> GSQVQTNVRCQGGSCASVCRRE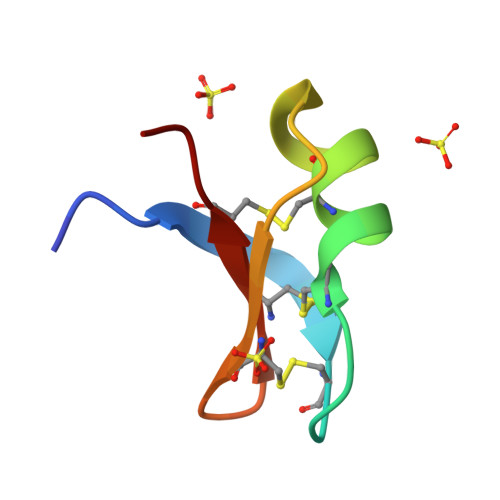IGVAAGRCINGRCVCYRN> STSDRLKAVEQNLYDVGPRDSGGREGPGHYIAISGNTAAGKTTLIETLAGSLRAAGADAVGVSERVFHHRYLKLMFSASADFAFPIQLSFMLERHLLLLDNLVRRGRTMVMERSHLDDAMFVREHVASGAITAAQQRAYTEVSGELNARIPNPDLIVLMNPEPE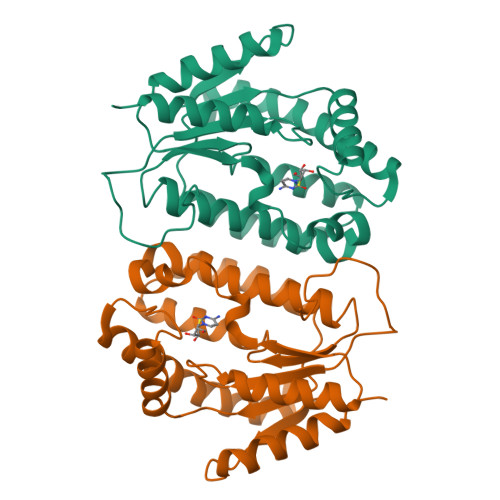LSLERLARAEAEGSRPREFPSDAAKRAWVHRWYDLYQELHDDYRRRAVDGDLRGTELLELDAAASPEEKIATVTARARSLVVG> ALDVRGGYRSGSHAYETRLKVSEGWQNGWWASMESNTWNTIHDNKKENAALNDVQVEVNYAIKLDDQWTVRPGMLTHFSSNGTRYGPYVKLSWDATKDLNFGIRYRYDWKAYRQQDLSGDMSRDNVHRWDGYVTYHINSDFTFAWQTTLYSKQNDYRYANHKKWATENAFVLQYHMTPDITPYIEYDYLDRQG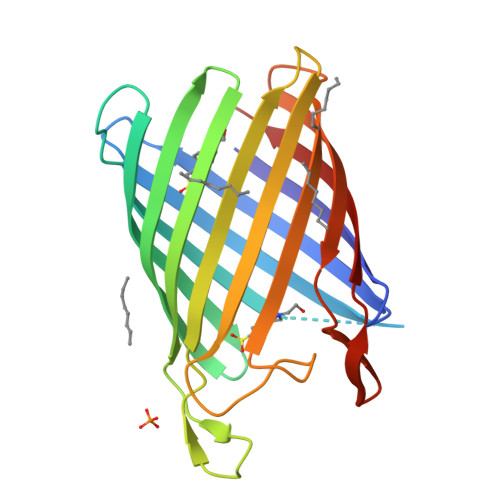VYNGRDNLSENSYRIGVSFKL>[2x]MAEDADMRNELEEMQRRADQLADESLESTRRMLQLVEESKDAGIRTLVMLDEQGEQLERIEEGMDQINKDMKEAEKNLTDLG;>ALSEIETRHSEIIKLENSIRELHDMFMDMAMLVE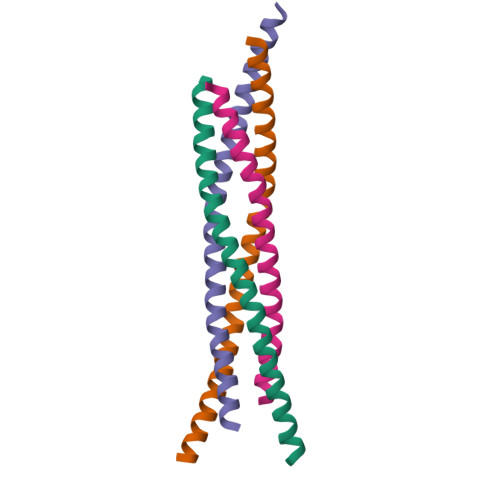SQGEMIDRIEYNVEHAVDYVERAVSDTKKAVKYQSKARRKKIM[2x]>MAEPWGNELASAAARGDLEQLTSLLQNNVNVNAQNGFGRTALQVMKLGNPEIARRLLLRGANPDLKDRTGFAVIHDAARAGFLDTLQTLLENQADVNIEDNEGNLPLHLAAKEGHLRVVEFLVKHTASNVGHRNHKGDTACDLARLYGRNEVVSLMQAN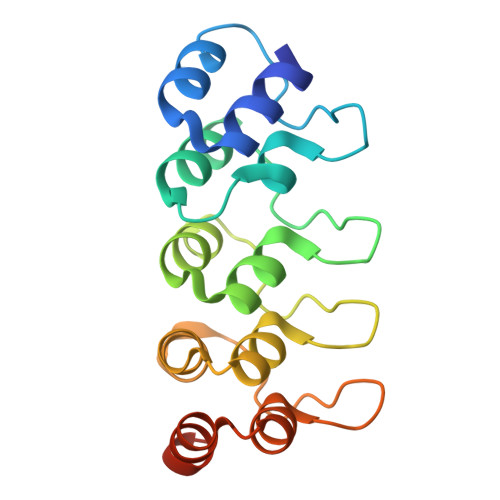GAGGATNLQ[2x]> MGGEVEKI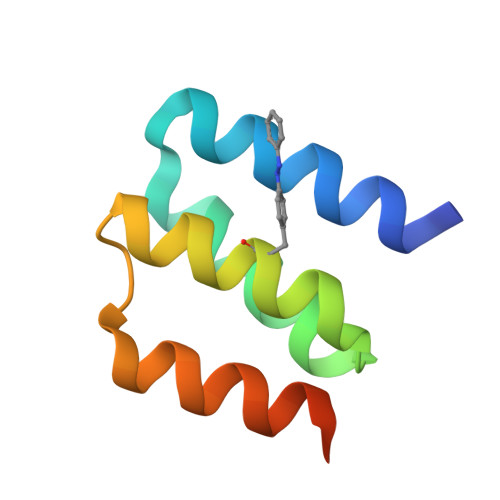VREAARAAREGDKEKLKELLAEAVAKGYVEATKFIAELALKAGAITKEEKAKYIAKAENGSHHHHHH> EWSYTGEHGTEHWGDSFATCAEGVNQTPIDINQTTQAELAPLHLDYEGQVTELVNNGHTIQANLTGKNTLTVDGKTFELKQFHFHTP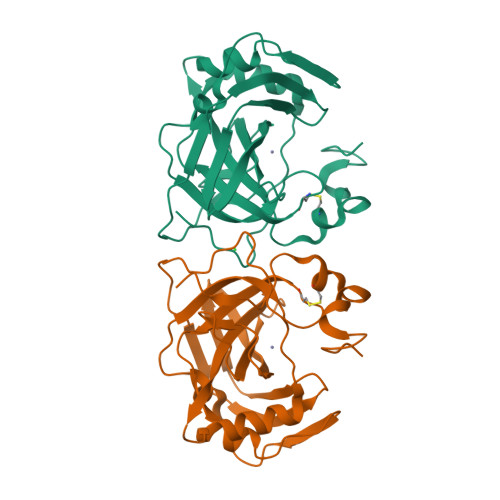SENYLKGKQYPLEAHFVHATDKGELAVVAVMFDFGPRSNNELTTLLASIPSKGQTVELKEALNPADLLPRDREYYRFNGSLTTPPCSEGVRWFVMQEPQTSSKAQTEKLQAVMGNNARPLQPLNARLILE>[6x]MVPVRMAVIADPETAQGFRLAGLEGYGASSAEEAQSLLET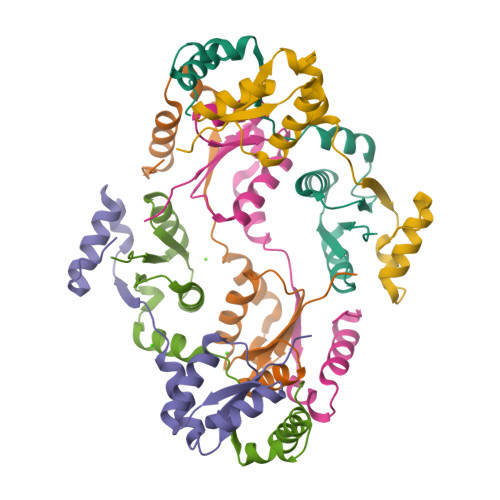LVERGGYALVAVDEALLPDPERAVERLMRGRDLPVLLPIAGLKEAFQGHDVEGYMRELVRKTIGFDIKL>GHMSLGSQKERLLDELTLEGVARYMQSERCRRVICLVGAGISTSAGIPDFRSPSTGLYDNLEKYHLPYPEAIFEISYFKKHPEPFFALAKELYPGQFKPTICHYFMRLLKDKGLLLRCYTQNIDTLERIAGLEQEDLVEAHGTFYTSHCVSASCRHEYPLSWMKEKIFSEVTPKCEDCQSLVKPDIVFFGESLPARFFSCMQSDFLKVDLLLVMGTSLQVQPFASLISKAPLSTPRLLINKEKAGQSDPFLGMIMGLGGGMDFDSKKAYRDVAWLGECDQGCLALAELLGWKKELEDLVRREHASIDAQS[2x]

Sirtuins constitute a family of NAD+-dependent enzymes that catalyse the cleavage of various acyl groups from the ∊-amino group of lysines. Sirtuins consist of a highly conserved catalytic deacylase domain of around 275 amino acids that is flanked by unstructured N- and C-termini that differ in their length and in their sequence. Of the seven members of the human sirtuin family, Sirt2 is mainly found in the cytoplasm, while Sirt3 is the main mitochondrial deacylase.

However, we succeeded using conventional screening methods and obtained crystals of both Sirt2 forms in complex with ADPR. Initially, Sirt250–356 crystallized in the presence of the cosubstrate NAD+ (2 mM) after a month in Index screen condition F10 (Hampton Research) with a 1:1 ratio of reservoir solution to protein solution at 4°C. This crystallization condition was optimized to 30%(w/v) PEG 3350, 0.2 M NaCl in 0.1 M bis-tris buffer at pH 6.25 and 4°C. Additionally, the NAD+ concentration and the protein:reservoir ratio were increased to 20 mM and 3:1, respectively. Each Sirt2 molecule contains the product analogue ADPR formed through the hydrolysis of NAD+. The structure of Sirt250–356 in complex with ADPR is very similar to the structure of Sirt2–ADPR recently published by Moniot et al., but everything is observed in greater detail. The asymmetric unit also contains two very similar monomers (r.m.s.d. of 0.19 Å for all Cα atoms) that adopt the ‘closed’ sirtuin conformation. However, the handling of the Sirt250–356 crystals turned out to be difficult and the crystals obtained were pseudo-merohedrally twinned. Additionally, we also provide an improved crystal structure of the Sirt2–ADPR complex.>[2x]SIEKIWAREILDSRGNPTVEVDLYTAKGLFRAAVPSGASTGIYEALELRDGDKQRYLGKGVLKAVDHINSTIAPALISSGLSVVEQEKLDNLMLELDGTENKSKFGANAILGVSLAVCKAGAAER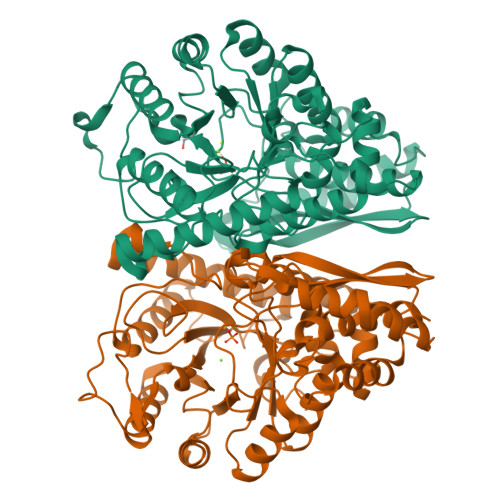ELPLYRHIAQLAGNSDLILPVPAFNVINGGSHAGNKLAMQEFMILPVGAESFRDAMRLGAEVYHTLKGVIKDKYGKDATNVGDEGGFAPNILENSEALELVKEAIDKAGYTEKIVIGMDVAASEFYRDGKYDLDFKSPTDPSRYITGDQLGALYQDFVRDYPVVSIEDPFDQDDWAAWSKFTANVGIQIVGDDLTVTNPKRIERAVEEKACNCLLLKVNQIGSVTEAIQACKLAQENGWGVMVSHRSGETEDTFIADLVVGLCTGQIKTGAPCRSERLAKYNQLMRIEEELGDEARFAGHNFRNPSVLHHHHHH> GSPSRAEYRNWSKPQCNITGFAPFSKDNSIRLSAGGDIWVTREPYVSCDPDKCYQFALGQGTTLNNGHSNDTVHDRTPYRTLLMNELGVPFHLGTKQVCIAWSSSSCHDGKAWLHVCVTGDDENATASFIYNGRLVDSIGSWSKKILRTQESECVCINGTCTVVMTDGSASGKADTKILFIEEGKIVHTSPLSGSAQHVEECSCYPRYPGVRCVCRDNWKGSNRPIVDINVKDYSIVSSYVCSGLVGDTPRKNDSSSSSHCLDPNNEEGGHGVKGWAFDDGNDVWMGRTISEKLRSGYETFKVIEGWSKPNSKLQINRQVIVDRGNRSGYSGIFSVEGKSCINRCFYVELIRGRKQETEV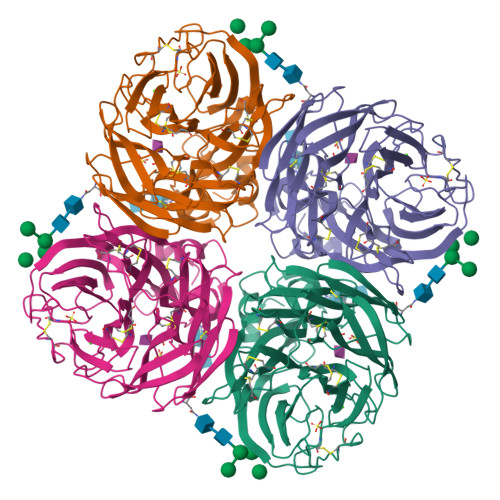LWTSNSIVVFCGTSGTYGTGSWPDGADINLMPI>[2x]MASLPILTVLEQSQVSPPPDTLGDKSLQLTFFDFFWLRSPPINNLFFYELPITRSQFTETVVPNIKHSLSITLKHFYPFVGKLVVYPAPTKKPEICYVEGDSVAVTFAECNLDLNELTGNHPRNCDKFYDLVPILGESTRLSDCIKIPLFSVQVTLFPNQGIAIGITNHHCLGD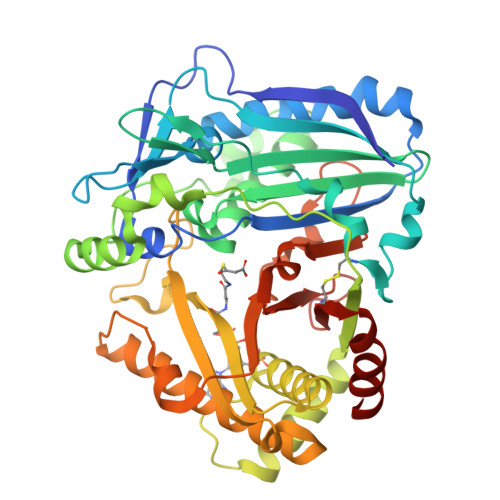ASTRFCFLKAWTSIARSGNNDESFLANGTRPLYDRIIKYPMLDEAYLKRAKVESFNEDYVTQSLAGPSDKLRATFILTRAVINQLKDRVLAQLPTLEYVSSFTVACAYIWSCIAKSRNDKLQLFGFPIDRRARMKPPIPTAYFGNCVGGCAAIAKTNLLIGKEGFITAAKLIGENLHKTLTDYKDGVLKDDMESFNDLVSEGMPTTMTWVSGTPKLRFYDMDFGWGKPKKLETVSIDHNGAISINSCKESNEDLEIGVCISATQMEDFVHIFDDGLKAYL>MKFAEHLSAHITPEWRKQYIQYEAFKDMLYSAQDQAPSVEVTDEDTVKRYFAKFEEKFFQTCEKELAKINTFYSEKLAEAQRRFATLQNELQSSLDAQKESTGVTTLRQRRKPVFHLSHEERVQHRNIKDLKLAFSEFYLSLILLQNYQNLNFTGFRKILKKHDKILETSRGADWRVAHVEVAPFYTCKKINQLISETEAVVTNELEDGDRQKAMKRLRVPPLGAAQPAPAWTTFRVGLFCGIFIVLNITLVLAAVFKLETDRSIWPLIRIYRGGFLLIEFLFLLGINTYGWRQAGVNHVLIFELNPRSNLSHQHLFEIAGFLGILWCLSLLACFFAPISVIPTYVYPLALYGFMVFFLINPTKTFYYKSRFWLLKLLFRVFTAPFHKVGFADFWLADQLNSLSVILMDLEYMICFYSLELKWDESKGLLPNNSEESGICHKYTYGVRAIVQCIPAWLRFIQCLRRYRDTKRAFPHLVNAGKYSTTFFMVTFAALYSTHKERGHSDTMVFFYLWIVFYIISSCYTLIWDLKMDWGLFDKNAGENTFLREEIVYPQKAYYYCAIIEDVILRFAWTIQISITSTTLLPHSGDIIATVFAPLEVFRRFVWNFFRLENEHLNNCGEFRAVRDISVAPLNADDQTLLEQMMDQDDGVRNR[2x];>[2x]VDERNECGQTPLMIAAEQGNLEIVKELIKNGANCNLEDLDNWTALISASKEGHVHIVEELLKCGVNLEHRDMGGWTALMWACYKGRTDVVELLLSHGANPSVTGLYSVYPIIWAAGRGHADIVHLLLQNGAKVNCSDKYGTTPLVWAARKGHLECVKHLLAMGADVDQEGANSMTALIVAVKGGYTQSVKEILKRNPNVNLTDKDGNTALMIASKEGHTEIVQ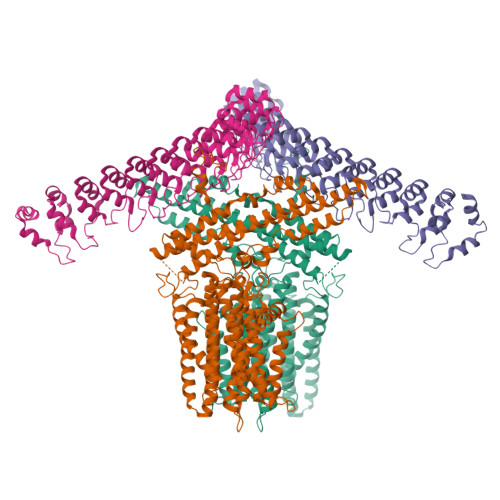DLLDAGTYVNIPDRSGDTVLIGAVRGGHVEIVRALLQKYADIDIRGQDNKTALYWAVEKGNATMVRDILQCNPDTEICTKDGETPLIKATKMRNIEVVELLLDKGAKVSAVDKKGDTPLHIAIRGRSRKLAELLLRNPKDGRLLYRPNKAGETPYNIDCSHQKSILTQIFGAR> DRWGSMNSLIKENMRMKVVLEGSVNGHQFKCTGEGEGNPYMGTQTMRIKVIEGGPLPFAFDILATSFMYGSRTFIKYPKGIPDFFKQSFPEGFTWERVTRYEDGGVITVMQDTSLEDGCLVYHAQVRGVNFPSNGAVMQKKTKGWEPNTEMMYPADGGLRGYTHMALKVDGGGHLSCSFVTTYRSKKTVGNIKMPGIHAVSHRLERLEESDNEMFVVQREHAVAKFAGLGGG

GECIs are prominent tools to monitor [Ca2+] in defined cells and intra-cellular compartments. To create a red GECI, we selected the red fluorescent protein (FP) mRuby (an engineered variant of eqFP611 exhibiting high thermodynamic stability and monomericity) and replaced cpEGFP with circularly permuted mRuby in the GCaMP3 scaffold. To aid our protein engineering efforts, we sought to solve the crystal structures of mRuby, RCaMP, and R-GECO1. High-resolution crystal structures of mRuby in several states, as well as a structure of a Ca2+-loaded RCaMP variant, aided optimization of the red GECI scaffold to useful performance levels.

Structural information on the parent protein of mRuby, eqFP611 (86% sequence identity with mRuby), has been published, however, no protein structure of mRuby was available at the time of initial RCaMP engineering, hampering optimization efforts. It has previously been shown that pH can have a large effect on chromophore conformation in red FPs; therefore we determined the crystal structure of mRuby at two different pHs: 4.5 and 8.5. The structure of mRuby at pH 8.5 shows a trans-isomer of the red 2-(iminomethyl)-4-(4-hydroxybenzylidene)-imidazol-5-one chromophore, while the structure at pH 4.5 shows a mixture of ~60% trans and ~40% cis. The large difference in pH had no notable effect on overall mRuby protein structure (RMSD = 0.13 Å for 208 Cα atoms). Similar pH-dependent cis-trans conformational changes also occur in the related FP eqFP578 (70% sequence identity with mRuby). Crystal structures of mRuby at low and high pH revealed a cis-trans chromophore isomerization in acidic environments. In contrast with the chromophore in the structure of mRuby crystallized at pH 8.5, the RCaMP structure (crystallized at pH 7.5) shows the (4-hydroxybenzylidene)-imidazol-5-one moiety of the chromophore to be a cis-isomer. Superimposition of both mRuby structures and the cp-mRuby domain of RCaMP demonstrates a slight (~1 Å) shift of the RCaMP chromophore (red structure in Figure 3C) relative to both isomers of the mRuby chromophore (cyan in Figure 3C).> GSQSAGGAMNTQIVPDAATCPACLAEMNTPGERRYRYPFINCTHCGPRFTIIRAMPYDRPFTVMAAFPLCPACDKEYRDPLDRRFHAQPVACPECGPYLEWVSHGEHAEQEAALQAAIAQLKMGNIVAIKGIGGFHLACDARNSNAVATLRARKHRPAKPLAVMLPVADGLPDAARQLLTTPAAPIVLVDKKYVPELCDDIAPGLNEVGVMLPANPLQHLLLQELQCPLVMTSGNLSGKPPAISNEQALEDLQGIADGFLIHNRDIVQRMDDSVVRESGEMLRRSRGYVPDALALPPGFKNVPPVLCLGAD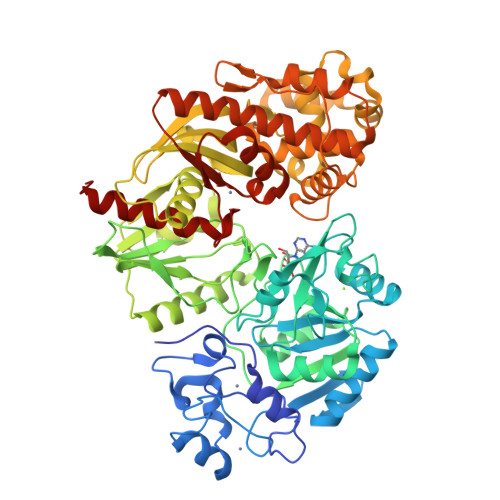LKNTFCLVRGEQVVLSQHLGDLSDDGIQTQWREALRLMQNIYNFTPQYVVHDAHPGYVSCQWASEMNLPTQTVLHHHAHAAACLAEHQWPLDGGDVIALTLDGIGMGENGALWGGECLRVNYRECEHLGGLPAVALPGGDLAAKQPWRNLLAQCLRFVPEWQNYPETASVAAANWSVLARAIERGINAPLASSCGRLFDAVAAALGCAPATLSYEGEAACALEALAASCDGVTHPVTMPRVDNQLDLATFWQQWLNWQAPVNQRAWAFHDALAQGFAALMREQATMRGITTLVFSGGVIHNRLLRARLAHYLADFTLLFPQSLPAGDGGLSLGQGVIAAARWLAGEV> HKTFVEKYEKQIKHFGMLRRWDDS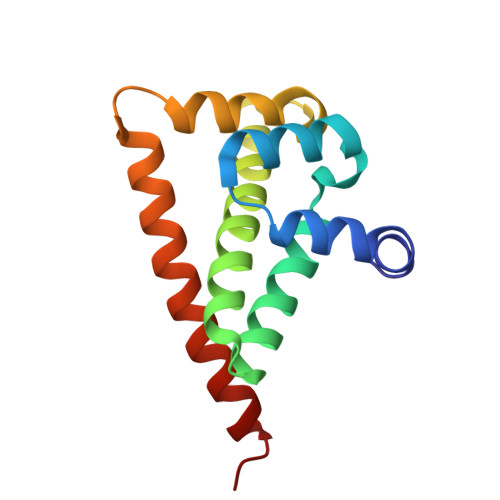QKYLSDNVHLVCEETANYLVIWCIDLEVEEKCALMEQVAHQTIVMQFILELAKSLKVDPRACFRQFFTKIKTADRQYMEGFNDELEAFKERVRGRAKLRIEKAMK>MVPISPIETVPVKLKPGMDGPKVKQWPLTEEKIKALVEICTEMEKEGKISKIGPENPYNTPVFACKKKDSTKWRKLVDFRELNKRTQDFWEVQLGIPHPAGLKKKKSVTVLDVGDAYFSVPLDEDFRKYTAFTIPSINNETPGIRYQYNVLPQGWKGSPAIFQSSMTKILEPFKKQNPDIVIYQYMDDLYVGSDLEIGQHRTKIEELRQHLLRWGLTTPDKKHQKEPPFLWMGYELHPDKWTVQPIVLPEKDSWTVNDIQKLVGKLNWASQIYPGIKVRQLSKLLRGTKALTEVIPLTEEAELELAENREILKEPVHGVYYDPSKDLIAEIQKQGQGQWTYQIYQEPFKNLKTGKYARMRGAHTNDVKQLTEAVQKITTESIVIWGKTPKFKLPIQKETWETWWTEYWQATWIPEWEFVNTPPLVKLWYQLEKEPIVGAETFYVDGAANRETKLGKAGYVTNKGRQKVVPLTNTTNQKTELQAIYLALQDSGLEVNIVTDSQYALGIIQAQPDKSESELVNQIIEQLIKKEKVYLAWVPAHKGIGGNEQVDKLVSA[2x];>[2x]MAHHHHHHALEVLFQ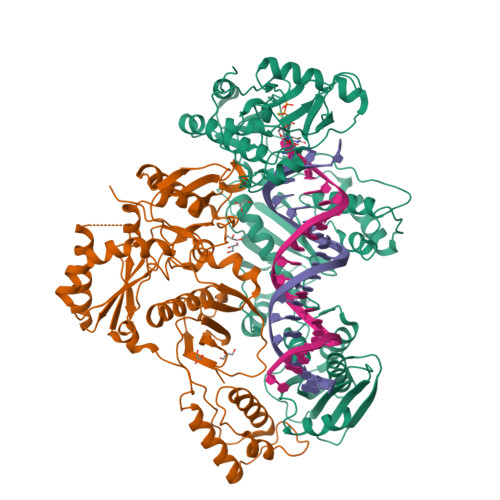GPISPIETVPVKLKPGMDGPKVKQWPLTEEKIKALVEICTEMEKEGKISKIGPENPYNTPVFAIKKKDSTKWRKLVDFRELNKRTQDFWEVQLGIPHPAGLKKKKSVTVLDVGDAYFSVPLDEDFRKYTAFTIPSINNETPGIRYQYNVLPQGWKGSPAIFQSSMTKILEPFKKQNPDIVIYQYMDDLYVGSDLEIGQHRTKIEELRQHLLRWGLTTPDKKHQKEPPFLWMGYELHPDKWTVQPIVLPEKDSWTVNDIQKLVGKLNWASQIYPGIKVRQLSKLLRGTKALTEVIPLTEEAELELAENREILKEPVHGVYYDPSKDLIAEIQKQGQGQWTYQIYQEPFKNLKTGKYARMRGAHTNDVKQLTEAVQKITTESIVIWGKTPKFKLPIQKETWETWWTEYWQATWIPEWEFVNTPPLVKLWYQ> ATPADWRSQSIYFLLTDRFARTDGSTTATCNTADQKYCGGTWQGIIDKLDYIQGMGFTAIWITPVTAQLPQTTAYGDAYHGYWQQDIYSLNENYGTADDLKALSSALHERGMYLMVDVVANHMGYDGAGSSVDYSVFKPFSSQDYFHPFCFIQNYEDQTQVEDCWLGDNTVSLPDLDTTKDVVKNEWYDWVGSLVSNYSIDGLRIDTVKHVQKDFWPGYNKAAGVYCIGEVLDGDPAYTCPYQNVMDGVLNYPIYYPLLNAFKSTSGSMDDLYNMINTVKSDCPDSTLLGTFVENHDNPRFASYTNDIALAKNVAAFIILNDGIPIIYAGQEQHYAGGNDPANREATWLSGYPTDSELYKLIASANAIRNY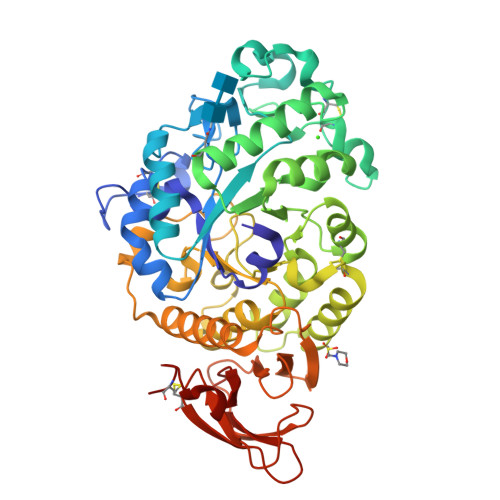AISKDTGFVTYKNWPIYKDDTTIAMRKGTDGSQIVTILSNKGASGDSYTLSLSGAGYTAGQQLTEVIGCTTVTVGSDGNVPVPMAGGLPRVLYPTEKLAGSKICS>MNPNQKIITIGSVCMTIGMANLILQIGNIISIWISHSIQLGNQNQIETCNQSVITYENNTWVNQTYVNISNTNFAAGQSVVSVKLAGNSSLCPVSGWAIYSKDNSVRIGSKGDVFVIREPFISCSPLECRTFFLTQGALLNDKHSNGTIKDRSPYRTLMSCPIGEVPSPYNSRFESVAWSASACHDGINWLTIGISGPDNGAVAVLKYNGIITDTIKSWRNNILRTQESECACVNGSCFTVMTDGPSNGQASYKIFRIEKGKIVKSVEMNAPNYHYEECSCYPDSSEITCVCRDNWHGSNRPWVSFNQNLEYQIGYICSGIFGDNPRPNDKTGSCGPVSSNGANGVKGFSFKYGNGVWIGRTKSISSRNGFEMIWDPNGWTGTDNNFSIKQDIVGINEWSGYS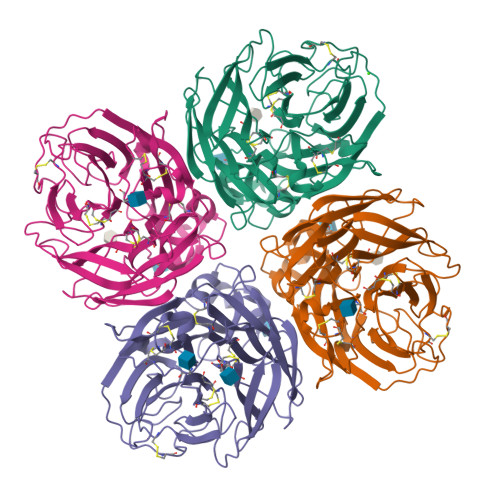GSFVQHPELTGLDCIRPCFWVELIRGRPKENTIWTSGSSISFCGVNSDTVGWSWPDGAELPFTIDK[4x]>[4x]GMNNKDLWIKEEIIWSEHKCIRFAAGGYEALIIPDVGGNVVELKDTNKGVTILRTPKKDLKFEDFKNRPQVYGLPVLFPPNRI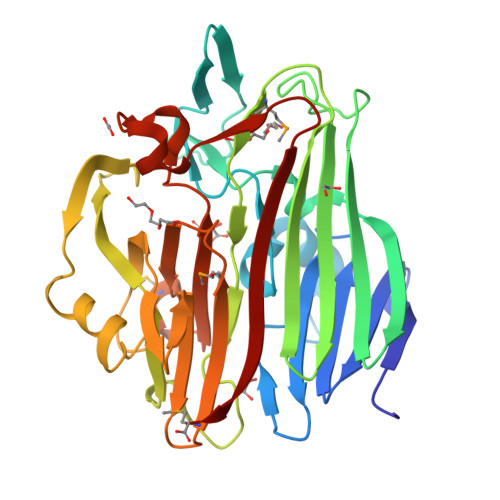DDGTFKLGDKTYKFPINEAKNNNYIHGFIKNSKWTVHKKKIDQDKALVEVVFDFTKENEAYKYFSHEFQFKLSYELSSKGLKQTTSVVNLSSEEMPLSVGYHSAFNVPFIEGSEDSNCRVKISIDKFWKQDSRNLPTGESFAPTGEQKEYLENGVAVASHPIESLFSLKDIDVNGKTFRGACIEDASKNTRVVYEMSSEYKYLVIWNDMGDKKYACIEPQTSIINSPNVKLDRSVSGFKTLKPNESWSGVCKLYIENM> MGAFLDKPKMEKHNAQGQGNGLRYGLSSMQGWRVEMEDAHTAVIGLPSGLESWSFFAVYDGHAGSQVAK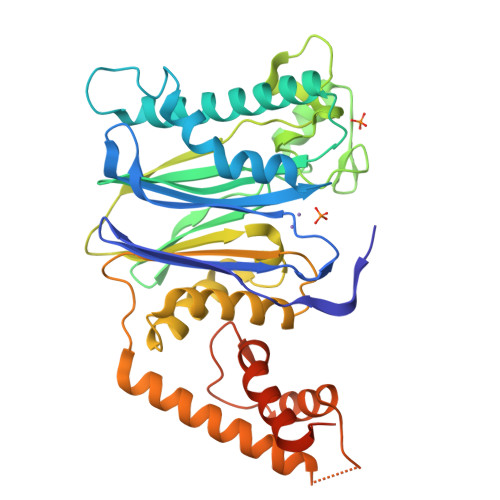YCCEHLLDHITNNQDFKGSAGAPSVENVKNGIRTGFLEIDEHMRVMSEKKHGADRSGSTAVGVLISPQHTYFINCGDSRGLLCRNRKVHFFTQDHKPSNPLEKERIQNAGGSVMIQRVNGSLAVSRALGDFDYKCVHGKGPTEQLVSPEPEVHDIERSEEDDQFIILACDGIWDVMGNEELCDFVRSRLEVTDDLEKVCNEVVDTCLYKGSRDNMSVILICFPNAPKVSPEAVKKEAELDKYLECRVEEIIKKQGEGVPDLVHVMRTLASENIPSLPPGGELASKRNVIEAVYNRLNPYKNDDTDSTSTDDMWLEHHHHHH>RECKTESNTFPGICITKPPCRKACISEKFTDGHCSKILRRCLCTKPC[14x]

NaD1, a plant defensin isolated from the flowers of the ornamental tobacco (Nicotiana alata), exhibits potent antifungal activity against pathogenic fungi, including Fusarium oxysporum, Botrytis cinerea, Aspergillus niger, Cryptococcus species, as well as the yeasts Saccharomyces cerevisiae and Candida albicans. The plant defensins are small (∼5 kDa, 45–54 amino acids), basic, cysteine-rich proteins that display a family-defining disulfide bond array (in a CI–CVIII, CII–CV, CIII–CVI, and CIV–CVII configuration) known as the cysteine-stabilized αβ (CSαβ) motif. This motif consists of a triple-stranded antiparallel β-sheet, which is cross-braced via three disulfide bonds at the core of the molecule to an α-helix (in a βαββ arrangement). NaD1 inhibits fungal growth in a three-stage process that involves specific interaction with the cell wall and entry into the cytoplasm before cell death.

The structure of monomeric NaD1 was used to solve the structure of a NaD1:PIP2 complex by molecular replacement and refined to a resolution of 1.6 Å with values of Rwork/Rfree of 0.155/0.184. Upon PIP2 binding, NaD1 forms an arch composed of 14 NaD1 molecules, with a final arch diameter of 90 Å and a width of 35 Å. Fourteen PIP2 molecules are bound in an extended binding groove on the inside of the arch. The observed NaD1:PIP2 oligomer can be described as an assembly of seven NaD1 dimers, which comprise two distinct NaD1:NaD1 interfaces. The first interface is formed by an antiparallel alignment of the β1-strand from each of two NaD1 molecules (monomers I and II) and exhibits two-fold symmetry between the associated monomers. It comprises an average buried surface area of 430 Å2 and is formed by a network of six hydrogen bonds involving R1, K4, E6, E27, K45, and C47. This dimeric arrangement leads to the formation of a ‘cationic grip’, which is able to accommodate two PIP2 head groups simultaneously. NaD1 binds PIP2 primarily via a ‘cationic grip’ that is created by a NaD1 dimer, which results in the formation of a distinct binding site formed by K4 together with residues 33–40, which comprise a characteristic ‘KILRR’ motif. PIP2 forms a dense network of hydrogen bonds involving K4, H33, K36, I37, L38, and R40 of a single NaD1 monomer. Bound PIP2 forms additional hydrogen bonds with R40 from monomer II and K36 from monomer IV′, with the full PIP2 binding site in the oligomer comprising contributions from three different NaD1 molecules. Examination of the PIP2 binding pockets in the NaD1:PIP2 oligomer suggests that R40, which contacts two adjacent PIP2 molecules simultaneously and interacts with the phosphate moiety at position 4, is critical for cooperative binding of PIP2 and therefore formation of the NaD1:PIP2 oligomer.TMEM16A is a member of the large TMEM16 family of membrane proteins, also known as anoctamins. Calcium-activated chloride channels (CaCCs) are important constituents of diverse physiological processes, ranging from epithelial chloride secretion to the control of electrical excitability in smooth muscles and neurons. These ligand-gated ion channels are activated upon an increase of the intracellular Ca2+ concentration as a consequence of cellular signaling events. Although it was initially anticipated that all TMEM16 proteins would function as anion channels, it is now generally accepted that only two family members (the closely related TMEM16A and B) are ion channels, whereas most others work as lipid scramblases, which catalyze the passive and bidirectional diffusion of lipids between the two leaflets of a phospholipid bilayer.

Here we have resolved this controversy by the structure determination of mouse TMEM16A (mTMEM16A) by cryo-electron microscopy (cryo-EM) at 6.6 Å resolution and a complementary electrophysiological characterization of pore mutants. For that purpose, we generated a stable HEK293 cell-line, which constitutively expresses the (ac) isoform of mTMEM16A, and purified the protein at a saturating calcium concentration in the detergent digitonin. Due to the presence of Ca2+, it likely shows the channel in a Ca2+-bound conformation. In light of the irreversible rundown of TMEM16A-mediated currents observed in patch-clamp experiments at high Ca2+ concentrations, it is at this point ambiguous whether this conformation corresponds to a conducting or a non-conducting state of the channel. The protein shows a similar overall fold and dimeric organization as the lipid scramblase nhTMEM16. Hence, the interaction of the subunits within the mTMEM16A dimer differs significantly from nhTMEM16 since the cytosolic domains do not contribute to the dimer interface. Instead, interactions are established mainly at the extracellular part of transmembrane α-helix 10, which is in a similar location as in nhTMEM16 but extends further towards the outside. The pore region of mTMEM16A, also containing the regulatory calcium-binding site, is formed by transmembrane α-helices 3–8. We could further constrain the position of the conserved calcium-binding site, as density between α-helices 6, 7 and 8 coincides with the position of the two bound calcium ions of nhTMEM16. As a consequence of conformational rearrangements, α4 and α6, which line the opposite borders of the membrane-accessible subunit cavity of nhTMEM16, have come into contact at the extracellular part of the membrane to form a protein-enclosed conduit that is shielded from lipids.

>MRVPEKYSTLPAEDRSVHIVNICAIEDLGYLPSEGTLLNSLSVDPDAECKYGLYFRDGKRKVDYILVYHHKRASGSRTLARRGLQNDMVLGTRSVRQDQPLPGKGSPVDAGSPEVPMDYHEDDKRFRREEYEGNLLEAGLELENDEDTKIHGVGFVKIHAPWHVLCREAEFLKLKMPTKKVYHISETRGLLKTINSVLQKITDPIQPKVAEHRPQTTKRLSYPFSREKQHLFDLTDRDSFFDSKTRSTIVYEILKRTTCTKAKYSMGITSLLANGVYSAAYPLHDGDYEGDNVEFNDRKLLYEEWASYGVFYKYQPIDLVRKYFGEKVGLYFAWLGAYTQMLIPASIVGVIVFLYGCATVDENIPSMEMCDQRYNITMCPLCDKTCSYWKMSSACATARASHLFDNPATVFFSVFMALWAATFMEHWKRKQMRLNYRWDLTGFEEEEEAVKDHPRAEYEARVLEKSLRKESRNKETDKVKLTWRDRFPAYFTNLVSIIFMIAVTFAIVLGVIIYRISTAAALAMNSSPSVRSNIRVTVTATAVIINLVVIILLDEVYGCIARWLTKIEVPKTEKSFEERLTFKAFLLKFVNSYTPIFYVAFFKGRFVGRPGDYVYIFRSFRMEECAPGGCLMELCIQLSIIMLGKQLIQNNLFEIGIPKMKKFIRYLKLRRQSPSDREEYVKRKQRYEVDFNLEPFAGLTPEYMEMIIQFGFVTLFVASFPLAPLFALLNNIIEIRLDAKKFVTELRRPVAIRAKDIGIWYNILRGVGKLAVIINAFVISFTSDFIPRLVYLYMYSQNGTMHGFVNHTLSSFNVSDFQNGTAPNDPLDLGYEVQICRYKDYREPPWSEHKYDISKDFWAVLAARLAFVIVFQNLVMFMSDFVDWVIPDIPKDISQQIHKEKVLMVELFMREEQGKQQLLDTWMEKEKPRDVPCNNHSPTTHPEAGDGSPVPSYEYHGDAL[2x]> MAWATTFYNVFVKRNSAFVATILASAFVFDMTFETAIDNFWDRINAGKQWKDIRHKYIEAAGDDD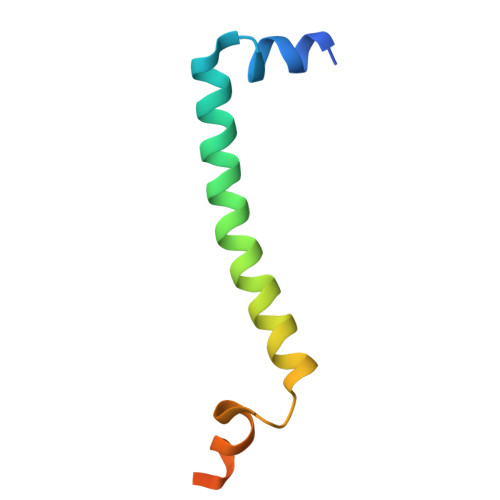EDD> PS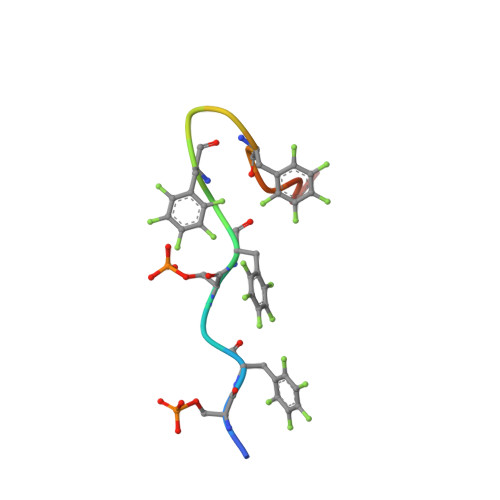FDSFDFEDFPAALWX(1R)-1,5-anhydro-1-(5-methyl-1,3-benzothiazol-2-yl)-D-glucitol | C14 H17 N O5 S | 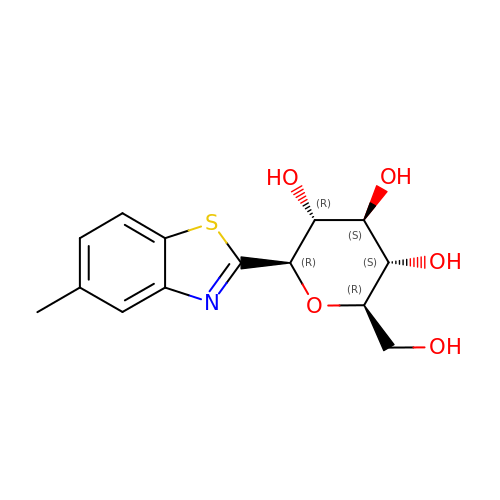WGJFWQVWYRZPEP-KABOQKQYSA-N> SKGLEDSSTISFITWNIDGLDGCNLPERARGVCSCLALYSPDVVF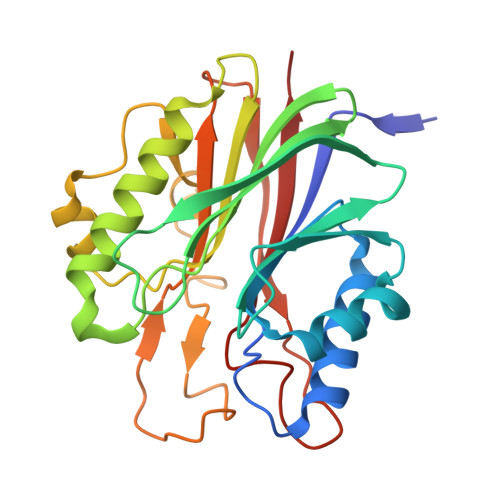LQEVIPPYCAYLKKRAASYTIITGNEEGYFTAILLKKGRVKFKSQEIIPFPNTKMMRNLLCVNVSLGGNEFCLMTSHLESTREHSAERIRQLKTVLGKMQEAPDSTTVIFAGDTNLRDQEVIKCGGLPDNVFDAWEFLGKPKHCQYTWDTKANNNLRIPAAYKHRFDRIFFRAEEGHLIPQSLDLVGLEKLDCGRFPSDHWGLLCTLNVVL> DPDTAVTNKQSFSTDVIYQVFTDRFLDGNPSNNPTGAAYDATCSNLKLYCGGDWQGLINKINDNYFSDLGVTALWISQPVENIFATINYSGVTNTAYHGYWARDFKKTNPYFGTMADFQNLITTAHAKGIKIVIDFAPNHTSPAMETDTSFAENGRLYDNGTLVGGYTNDTNGYFHHNGGSDFSSLENGIYKNTYDLADFNHNNATIDKYFKDAIKLWLDMGVDGIRVDAVKHMPLGWQKSWMSSIYAHKPVFTFGEWFLGSAASDADNTDFANKSGMSLLDFRFNSAVRNVFRDNTSNMYALDSMINSTATDYNQVNDQVTFIDNHDMDRFKTSAVNNRRLEQALAFTLTSRGVPAIYYGTEQYLTGNGDPD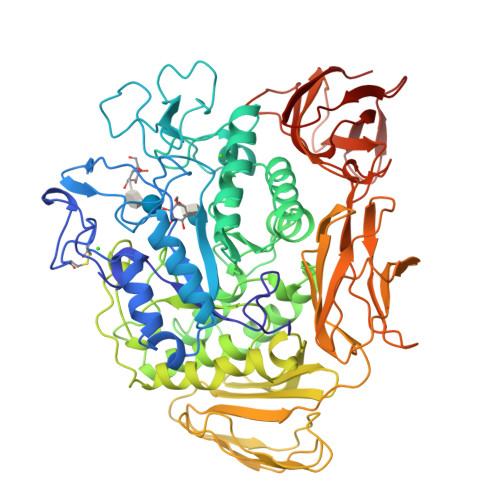NRAKMPSFSKSTTAFNVISKLAPLRKSNPAIAYGSTQQRWINNDVYVYERKFGKSVAVVAVNRNLSTSASITGLSTSLPTGSYTDVLGGVLNGNNITSTNGSINNFTLAAGATAVWQYTTAETTPTIGHVGPVMGKPGNVVTIDGRGFGSTKGTVYFGTTAVTGAAITSWEDTQIKVTIPSVAAGNYAVKVAASGVNSNAYNNFTILTGDQVTVRFVVNNASTTLGQNLYLTGNVAELGNWSTGSTAIGPAFNQVIHQYPTWYYDVSVPAGKQLEFKFFKKNGSTITWESGSNHTFTTPASGTATVTVNWQ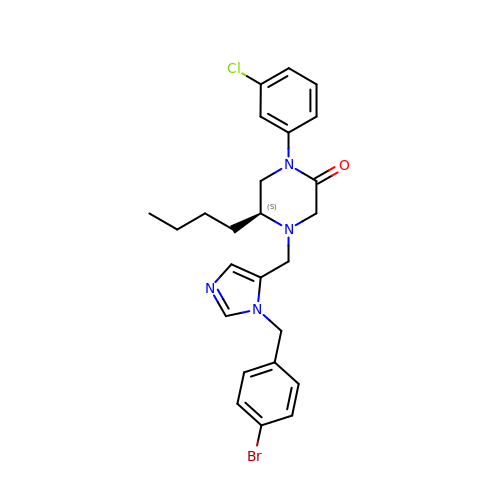(5S)-4-({1-[(4-bromophenyl)methyl]-1H-imidazol-5-yl}methyl)-5-butyl-1-(3-chlorophenyl)piperazin-2-one | C25 H28 Br Cl N4 O | DJAYAIKODCJWBJ-QHCPKHFHSA-N> ATLDSWLSNEATVARTAILNNIGADGAWVSGADSGIVVASPSTDNPDYFYTWTRDSGLVIK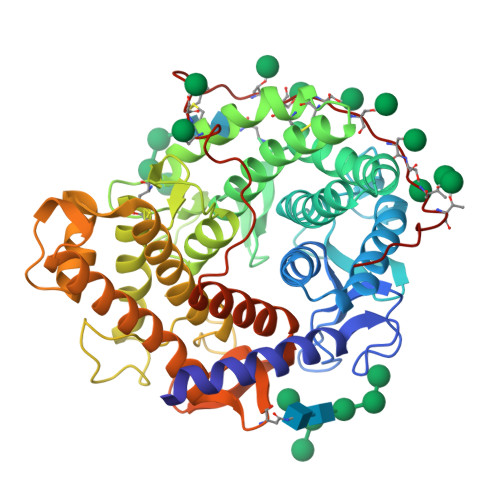TLVDLFRNGDTDLLSTIEHYISSQAIIQGVSNPSGDLSSGGLGEPKFNVDETAYTGSWGRPQRDGPALRATAMIGFGQWLLDNGYTSAATEIVWPLVRNDLSYVAQYWNQTGYDLWEEVNGSSFFTIAVQHRALVEGSAFATAVGSSCSWCDSQAPQILCYLQSFWTGSYILANFDSSRSGKDTNTLLGSIHTFDPEAGCDDSTFQPCSPRALANHKEVVDSFRSIYTLNDGLSDSEAVAVGRYPEDSYYNGNPWFLCTLAAAEQLYDALYQWDKQGSLEITDVSLDFFKALYSGAATGTYSSSSSTYSSIVSAVKTFADGFVSIVETHAASNGSLSEQFDKSDGDELSARDLTWSYAALLTANNRRNSVVPPSWGETSASSVPGTCAATSASGTYSSVTVTSWPSIVA> MAMKTQRKENVLFQNVKPREIPLVDNPFSTYPYKHVITETQPTQAKNQAIWGLVQMGLSG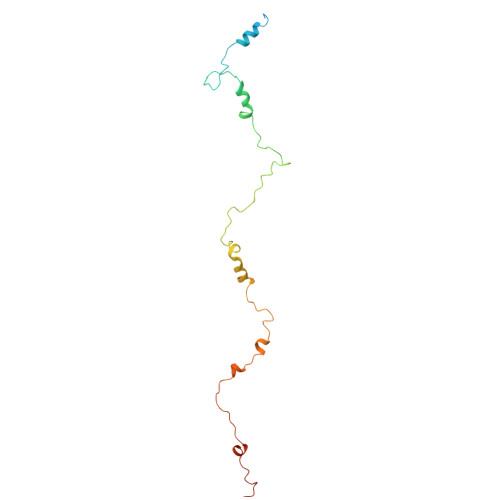EAAAMYGDVVVQKTTRACRKSEGGFKDVNTELWGTSPYLGRGDGEVYNMPASNQLLRGFESSLRGSRVRTQIDDKSFIPYTWQMIDVPLAAAKTSFIAGLDTRQQLAYGNP>MTTGKPNILIIMVDQLNGKLFPDGPADFLHAPNLKALAKRSARFHNNYTSSPLSAPARASFMAGQLPSRTRVYDNAAEYQSSIPTYAHHLRRAGYYTALSGKMHLVGPDQLHGFEERLTTDIYPADFGWTPDYRKPGERIDWWYHNLGSVTGAGVAEITNQMEYDDEVAFLANQKLYQLSRENDDESRRPWCLTVSFTHPHDPYVARRKFWDLYEDCEHLTPEVGAIPLDEQDPHSQRIMLSCDYQNFDVTEENVRRSRRAYFANISYLDEKVGELIDTLTRTRMLDDTLILFCSDHGDMLGERGLWFKMNFFEGSARVPLMIAGPGIAPGLHLTPTSNLDVTPTLADLAGISLEEVRPWTDGVSLVPMVNGVERTEPVLMEYAAEASYAPLVAIREGKWKYVYCALDPEQLFDLEADPLELTNLAENPRGPVD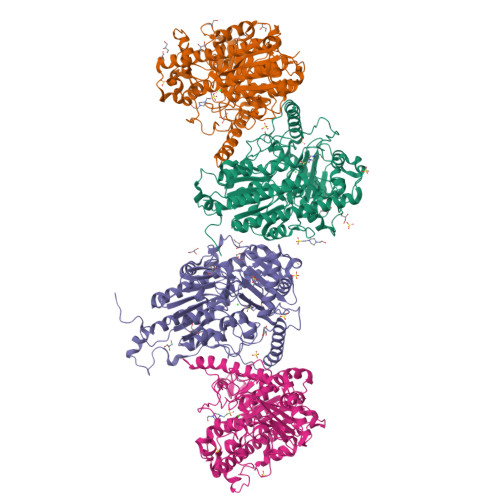QATLTAFRDMRAAHWDMEAFDAAVRESQARRWVVYEALRNGAYYPWDHQPLQKASERYMRNHMNLDTLEESKRYPRGEGSHHHHHH[4x]> MLRRSLLAFPWWNFQTEHRQRCVLMYGGARTKNTHNANHRVFIKKYKRNAFPNRTRHHWA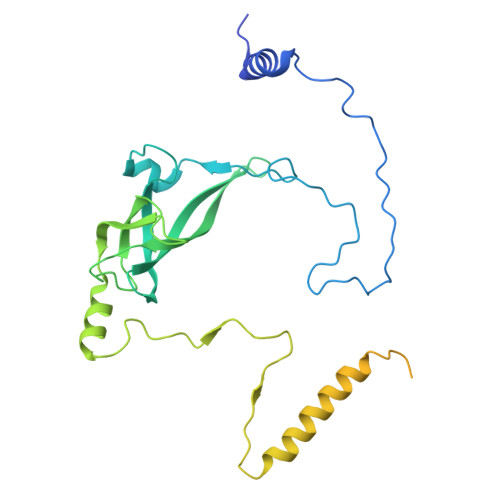VSMTGVLSQRPRRMPWPYDLTSLIFNQPRQGSDKIGYVVGTSMLKTAVVATNHMVYYPKFNQRVSRTKRFFAHDEDLACVEGDLVHIKQCRKISKYKHYYVFSILEPNVEGRERLKLGLKAVPPPLFGYPVSRRIVKLNLTSTEGTQEKLAAAIQEHVQDAYRFSGPTPDQPRNRLADPVTFEDANNMIAPNAPAAAALDASDSPPLLDRGEYTEVEQDTRNKKGDDYWMNLQPKEKYDFKSFKKSPRPLEDQVDPRLIDGKYDIPTTASENLYFQ> QAEEWYFGKITRRESERLLLNPENP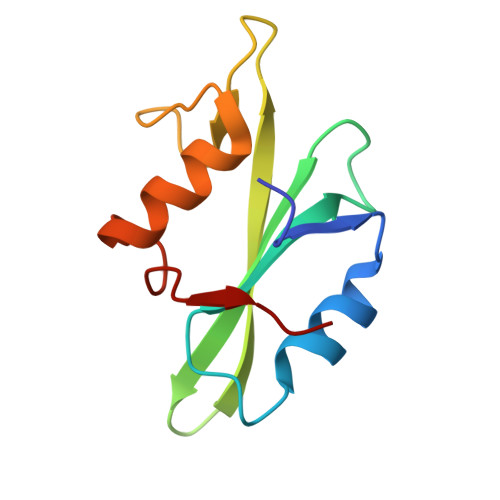RGTFLVRESETTKGAYCLSVSDFDNAKGLNVKHYKIRKLDSGGFYITSRTQFSSLQQLVAYYSKHADGLCHRLTNVCPT4-bromo-N-((1S,2R)-2-(naphthalen-1-yl)-1-(5-oxo-4,5-dihydro-1,3,4-oxadiazol-2-yl)propyl)benzenesulfonamide | C21 H18 Br N3 O4 S | 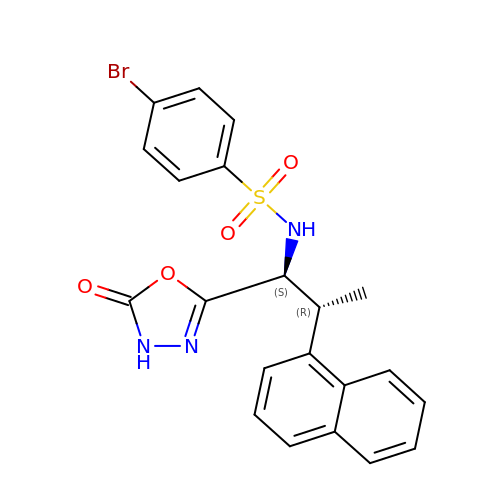RXRDLPNXTGZSLC-YJYMSZOUSA-N> MADPKKVLDKAKDEAENRVRELKQRLEELYKEARKLDLTQEMRQELVDKARAASLQANGDIFYAILRALAEA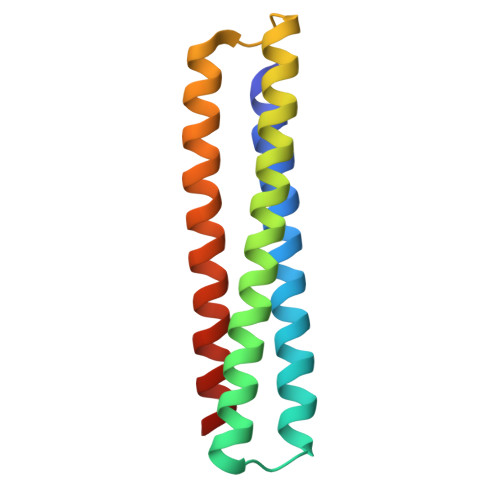EKLKKAGLVNSQQLDELKRRLEELAEEARRKAEKLRDEFRLKLEYG> GSMTSTVEFINRWQRIALLSQSLLELAQRG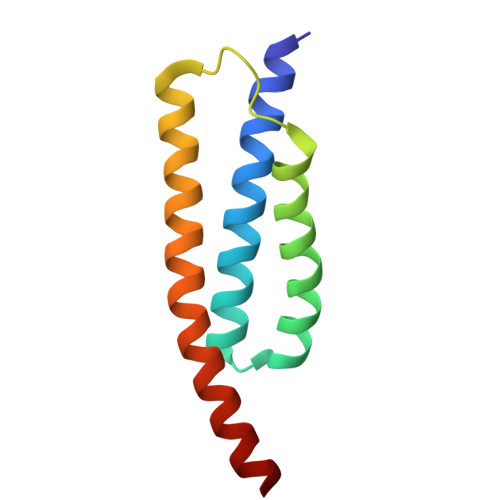EWDLLLQQEVSYLQSIETVMEKQTPPGITRSIQDMVAGYIKQTLDNEQLLKGLLQQRLDELSSLIG> EAEAEFNSINACLAAADVEFHEEDSEGWDMDGTAFNLRVDYDPAAIAIPRSTEDIAAAVQCGLDAGVQISAKGGGHSYGSYGFGGEDGHLMLELDRMYRVSVDDNNVATIQGGARLGYTALELLDQGNRALSHGTAPAVGVGGHVLGGGYGFATHTHGLTLDWLIGATVVLADASIVHVSETENADLFWALRGGGGGFAIVSEFEFNTFEAPEIITTYQVTTTWNRKQHVAGLKALQDWAQNTMPRELSMRLEINANALNWEGNFFGNAKDLKKILQPIMKKAGGKSTISKLVETDWYGQINTYLYGADLNITYNYDVHEYFYANSLTAPRLSDEAIQAFVDYKFDNSSVRPGRGWWIQWDFHGGKNSALAAVSNDETAYAHRDQLWLWQFYDSIYDYENNTSPYPESGFEFMQGFVATIEDTLPEDRKGKYFNYADTTLTKEEAQKLYWRGNLEKLQAIKAKYDPEDVFGNVVSVEPIAYLEQKLISEE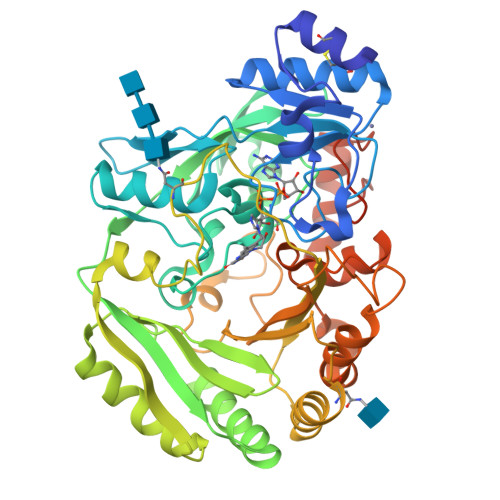DLNSAVDHHHHHH(2S)-2-{[(R)-{[(2R,3S,4R,5R)-5-(6-amino-9H-purin-9-yl)-3,4-dihydroxyoxolan-2-yl]methoxy}(hydroxy)phosphoryl]amino}-5-carbamimidamidopentanoic 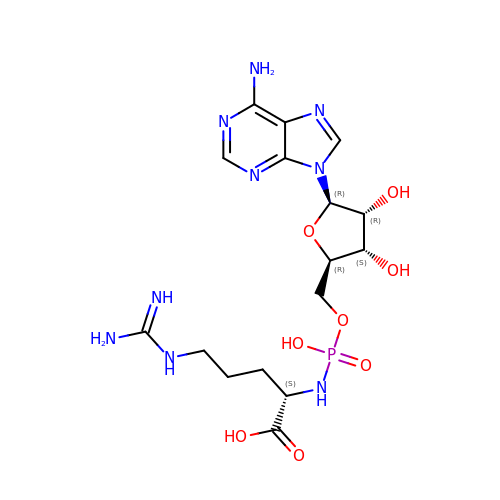acid (non-preferred name) | C16 H26 N9 O8 P | AXUGFAXGFGAXFD-TWBCTODHSA-N(7~{S})-2-(4-bromanyl-3,5-dimethoxy-phenyl)-7-(1-propanoylpiperidin-4-yl)-4,5,6,7-tetrahydropyrazolo[1,5-a]pyrimidine-3-carboxamide 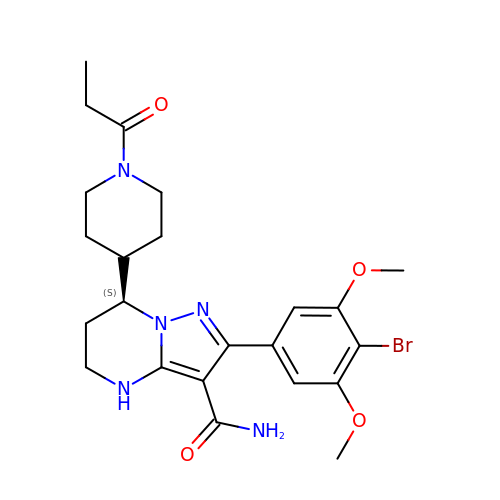| C23 H30 Br N5 O4 | GQJVVSVHZDAEOE-HNNXBMFYSA-N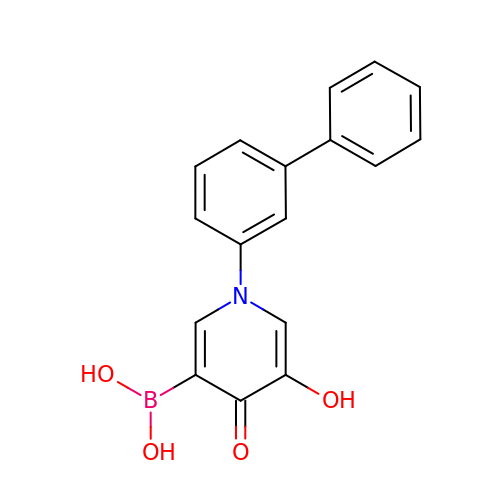[1-(biphenyl-3-yl)-5-hydroxy-4-oxo-1,4-dihydropyridin-3-yl]boronic acid | C17 H14 B N O4 | RJVMGRMKRJSOAH-UHFFFAOYSA-N> GSASCLELALEGERLCKSGDCRAGVSFFEAAVQVGTEDLKTLSAIYSQLGNAYFYLHDYAKALEYHHHDLTLARTIGDQLGEAKASGNLGNTLKVLGNFDEAIVCCQRHLDISRELNDKVGEARALYNLGNVYHAKGKSFGCPGPQDTGEFPEDVRNALQAAVDLYEENLSLVTALGDRAAQGRAFGNLGNTHYLLGNFRDAVIAHEQRLLIAKEFGDKAAERRAYSNLGNAYIFLGEFETASEYYKKTLLLARQLKDRAVEAQSCYSLGNTYTLLQDYEKAIDYHLKHLAIAQELKDRIGEGRACWSLGNAYT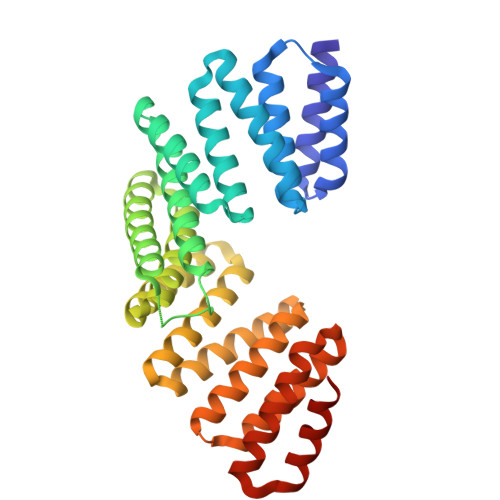ALGNHDQAMHFAEKHLEISREVGD> MAHHHHHHMRSPHIGQGSNSANVRRYNERLLLKTLRRAGSASKADLARLANMTGTAVGSIIASLADAKLIEFAGRTEGQRGQPASLIRLDPRGAFGIGVHLDRMRIETALVNFAGDVLGRRSHDTLLPPPAEVIEIVRHDIDAMQALLPAHERARLAGVGVAQPYNLGAWMRELGL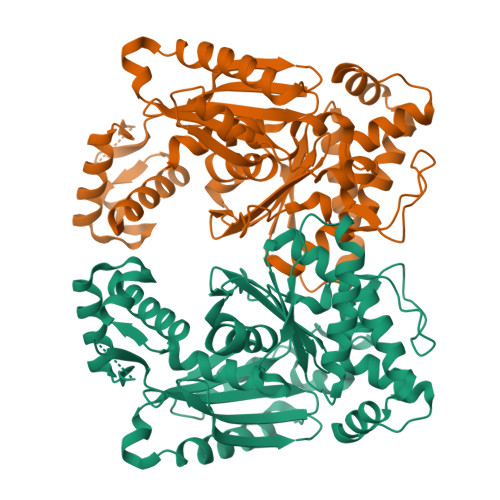APDTFRAWEDVDFASDLGRTVSLPVFGENDGNAAAIAELFYGYGRQCDDFVYLFIGPAIGGGIAIDGDCLRGVTGNAGDIAMIPVLPSRLASAPPPRGPWDILLARASLHALVRHLRHHGETVESRADLEACIARGLPAVTEWIDDCVDALAPALRAVLCVVDAPVVVLDADTDAGLLDALTSRLRAALVATAPEARGTPTLVRGTFGADAGAIGAATLPMYFNFSPRAGILRGARIESQEVNHVAI BD-FAE, a previously unknown protein encoded in a metagenomic PUL from beaver droppings belongs to the functionally diverse α/β-hydrolase superfamily. We demonstrated that BD-FAE removes feruloyl and acetyl groups from simple model substrates, acetyl groups from birchwood glucuronoxylan, and feruloyl groups from highly substituted AcFaXOS from corn fiber. The His-tag was not visible and the N-terminal tail showed weaker electron density than other residues of the protein, most likely due to its flexible protruding nature. Overall, the BD-FAE crystal structure adopted a typical α/β-hydrolase fold, which was consistent with the above mentioned BLASTp results. The active center contained the conserved catalytic triad of Ser128, Asp237 and His269 and the oxyanion hole was composed of NH-groups of Gly53 and Ser128.

The BD-FAE structure belonged to space group P43212 and contained one molecule in an asymmetric unit. The final model of BD-FAE was refined to 2.06 Å resolution and it contained the residues from Gln2 to Glu292. In the crystal structure of BD-FAE, a sulfate ion was bound to the active site, which originated most likely from the ammonium sulfate containing crystallization solution. It mimicked the binding of an acetyl group to the catalytic triad. Looking at the surface model it can be seen that the active site was solvent exposed and formed a shallow furrow. The N-terminal tail (Gln2-Pro7) protruded out of the core protein and packed against an adjacent symmetry molecule in the crystal. Such crystal packing did not form a closed-ended dimer but an unusual fourfold spiral shaped polymer, in which the active sites pointed to the center of the spiral. The interaction area of sequential molecules within the polymer was determined using PISA server and revealed 1055 Å2, which was typical for strong intermolecular interactions. In crystals of BD-FAE, the protruding N-terminal tail packed as a β-strand against a small β-sheet on the surface of another molecule, leading to an unusual fourfold spiral shaped polymer.

> MQDFQMPKGPAEDTYSTSWTNVNYASDSLESHNLDIYLPKEQKTAYKAIIIIYGSAWFANNAKAMASASIGAPLLKAGFAVISINHRSSMEAIWPAQIQDVKAAIRYVRSNAAKYNIDPSFIGITGFSSGGHLSAFAGVTNGVKTLTSGDLTVDIEGSLGNYLSTGSHVDAVVDWFGPVDMAHMSNCVAPNDASTPEAVLIGKKDPREEPDWVKLISPINFVDKDDPDILIIHGDADNVVPHCQSVNLKNVYDNAGAKATFISVPGGGHGPGCFDTQYFKDMTDFFTEQSTKLEHHHHHH> MRRSAWVFVAPWVPPPRHDVKVTMPPPPGGEVGGSYGVSTGYSDRLARTPYWKRMALSTYALRMKENETRYPMSPHREGEYDLRYTVTAYPDHIKHRPLLEIGEAHQIPT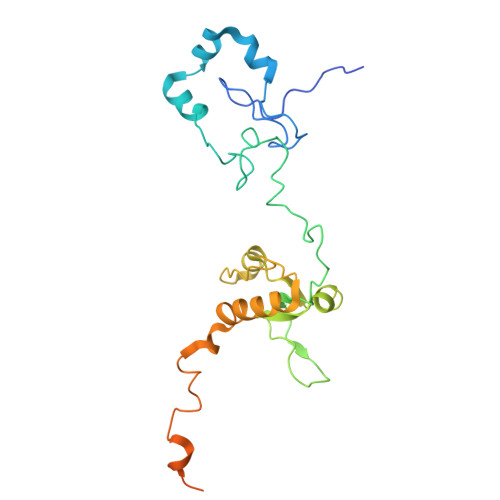IEIPVIFLVNLWDEERLTWFGRQYETVYVNRNVAREELLPQRYAIYATEEAYKLLGLPVVNHSIHEEIPKTPHAYKKLLEKQSYTEERWKYTIEYLFRKYEADPPELQDKSEDGWDGVEELATSATAGGAGDSLAKRKGPVKQRKARKIKLF3-(quinolin-2-yl)propanoic acid | C12 H11 N O2 | 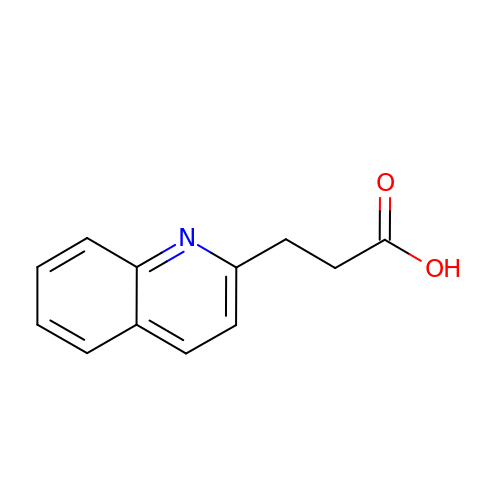PBXJDATXARPDPW-UHFFFAOYSA-N> MSLAKVWMYASWIPRGIPKAMANELSSAAAALAHPEAIARVAQLESQGKNPYRVARAEFWQMYLACWPYRFRNTVVEWETCKAKVLKGSVDLQDIVDLLYLLAWAYLFWIL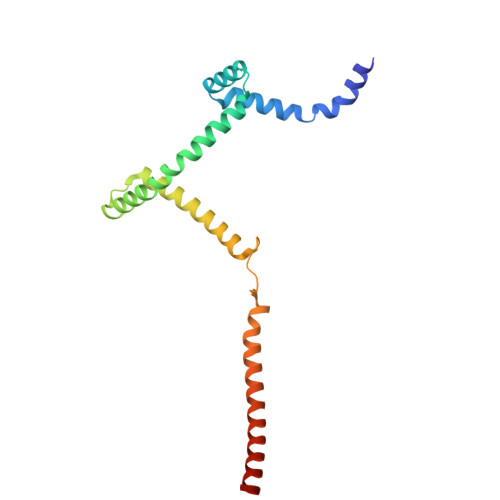GEIYGRGSLYGYRFDGEIHRQEAQNVILYKEKEAQEMAVVMEKLEKEIQEWLKTMEQE(2S)-2-azanyl-2-cyclopropyl-2-(4-phosphonophenyl)ethanoic acid | C11 H14 N O5 P | 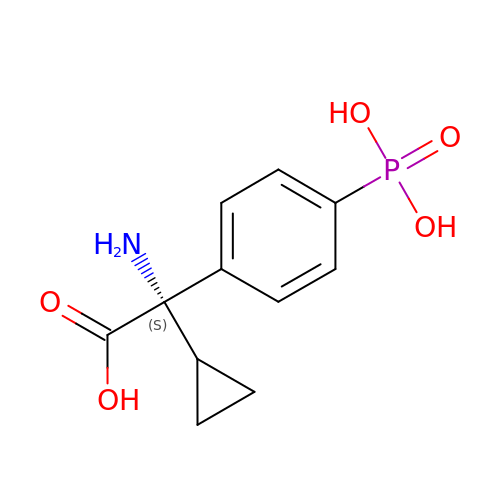IGODGTDUQSMDQU-NSHDSACASA-N> MNDIAHNLAQVRDKISAAATRCGRSPEEITLLAVSATAPASAIAEAIDAGQRQFGENYVQEGVDKIRHFQELGVTGLEWHFIGPLQSNKSRLVAEHFDWCHTIDRLRIATRLNDQRPAELPPLNVLIQINISDENSKSGIQLAELDELAAAVAELPRLRLRGLMAIPAPESEYVRQFEVARQMAVAFAGLKTRYPHIDTLSLGMSDDMEAAIAAGSTMVRIGTAIFGARDYSKK

The pyridoxal 5′‐phosphate (PLP) homeostasis protein (PLPHP) is a ubiquitous member of the COG0325 family with apparently no catalytic activity. Although the actual cellular role of this protein is unknown, it has been observed that mutations of the PLPHP encoding gene affect the activity of PLP‐dependent enzymes, B6 vitamers and amino acid levels. Here we report a detailed characterization of the Escherichia coli ortholog of PLPHP (YggS) with respect to its PLP binding and transfer properties, stability, and structure. YggS binds PLP very tightly and is able to slowly transfer it to a model PLP‐dependent enzyme, serine hydroxymethyltransferase.

We serendipitously discovered that the K36A variant of YggS, affecting the lysine residue that binds PLP at the active site, is able to bind PLP covalently. This observation led us to recognize that a number of lysine residues, located at the entrance of the active site, can replace Lys36 in its PLP binding role.> MGSSHHHHHHSQDPNSSSARLQVDKLFCFNILCVGETGIGKSTLMDTLFNTKFESDPATHNEPGVRLKARSYE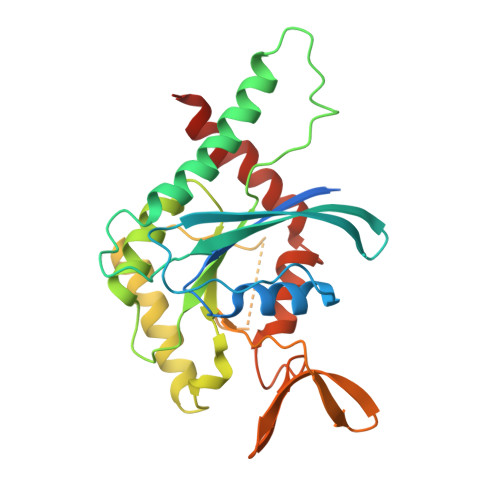LQESNVRLKLTIVDTVGFGDQINKDDSYKPIVEYIDAQFEAYLQEELKIKRSLFNYHDTRIHACLYFIAPTGHSLKSLDLVTMKKLDSKVNIIPIIAKADTIAKNELHKFKSKIMSELVSNGVQIYQFPTDEETVAEINATMSVHLPFAVVGSTEEVKIGNKMAKARQYPWGVVQVENENHCDFVKLREMLIRVNMEDLREQTHTRHYELYRRCKLEEMG>MGSSHHHHHHSSGLVPRGSGSDPTRKQKVEAQKQAEKLMKQIGVKNVKLSEYEMSIAAHLVDPLNMHVTWSDIAGLDDVITDLKDTVILPIKKKHLFENSRLLQPPKGVLLYGPPGCGKTLIAKATAKEAGCRFINLQPSTLTDKWYGESQKLAAAVFSLAIKLQPSIIFIDQIDSFLRNRSSSDHEATAMMKAQFMSLWDGLDTDHSCQVIVMGATNRPQDLDSAIMRRMPTRFHINQPALKQREAILKLILKNENVDRHVDLLEVAQETDGFSGSDLKEMCRDAALLCVREYVNSTSE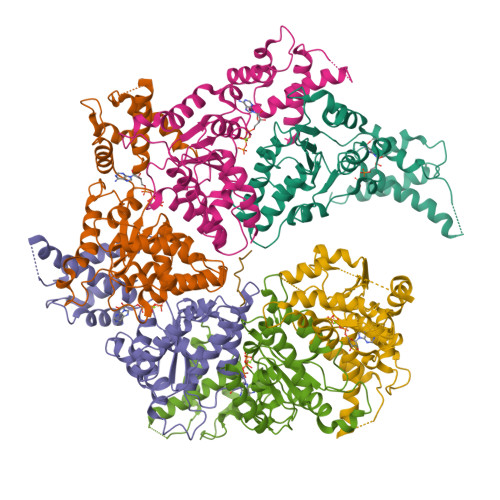ESHDEDEIRPVQQQDLHRAIEKMKKSKDAAFQNVLTHVCLD[6x]(2S,5R)-N-(2-aminoethoxy)-1-formyl-5-[(sulfooxy)amino]piperidine-2-carboxamide | C9 H18 N4 O7 S | 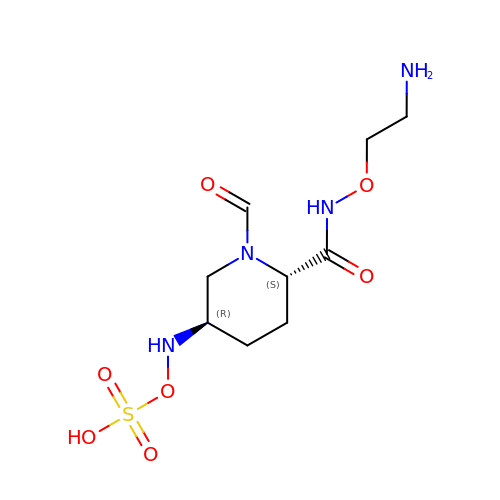YTAWXXHGLPATIN-SFYZADRCSA-N> QQQHK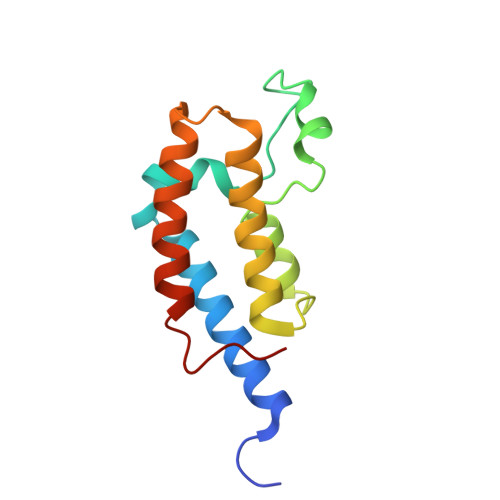VLKTVKVTEQLKHCSEILKEMLAKKHLPYAWPFYNPVDADALGLHNYYDVVKNPMDLGTIKGKMDNQEYKDAYEFAADVRLMFMNCYKYNPPDHEVVAMARTLQDVFELHFAKIPDEPIES>LEHHHHHHMALSAEGSSGGSRGGSPKAEAASVPSWPQILGRLTDNRDLARGQAAWAMDQIMTGNARPAQIAAFAVAMTMKAPTADEVGELAGVMLSHAHPLPADTVPDDAVDVVGTGGDGVNTVNLSTMAAIVVAAAGVPVVKHGARAASSLSGGADTLEALGVRIDLGPDLVARSLAEVGIGFCFAPRFHPSYRHAAAVRREIGVPTVFNLLGPLTNPARPRAGLIGCAFADLAEVMAGVFAARRSSVLVVHGDDGLDELTTTTTSTIWRVAAGSVDKLTFDPAGFGFARAQLDQLAGGDAQANAAAVRAVLGGARGPV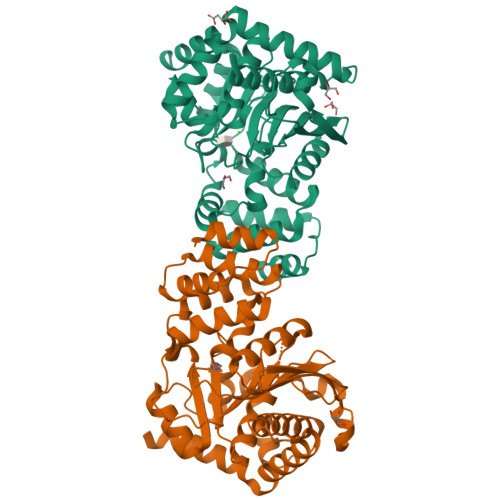RDAVVLNAAGAIVAHAGLSSRAEWLPAWEEGLRRASAAIDTGAAEQLLARWVRFGRQI[2x]4-{[(3S)-3-(5-methyl-2,4-dioxo-3,4-dihydropyrimidin-1(2H)-yl)piperidin-1-yl]sulfonyl}-2-(3-methylphenoxy)benzoic 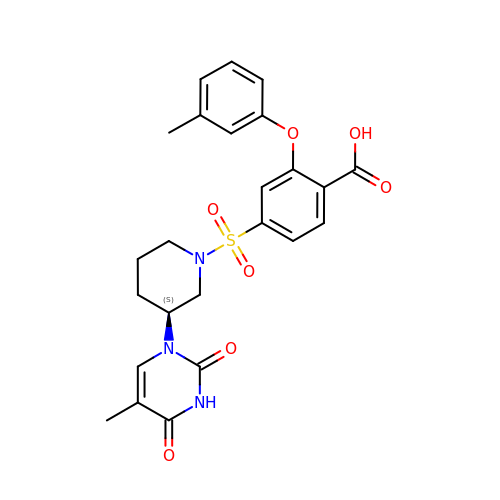acid | C24 H25 N3 O7 S | HYOKWKXYBOKTDO-KRWDZBQOSA-N> MTCQVTQKAREGTINPIFTCQPAGAQFASIGIKDCIGIVHGGQGCVMFVRLL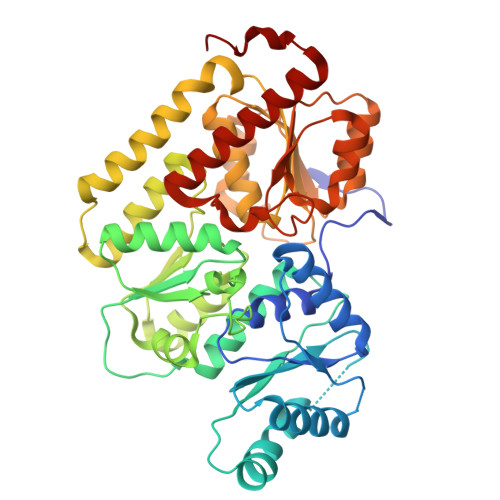ISQHMKESFEIASSSVHEDGAVFGALDRVETAVEVLLTRYPDVKVVPIITTCSTEIIGDDVDGLLSKLEDELLPTKFPGREVHLLTVHCPSFVGSMITGYDKAVHDFVKKFATKDEPSDKINLITGWVNPGDVKELKHLLEVMEVKANVLFEVESFDSPLMPDLEHHSHGSTTIEDLRDTANAKGTIALNRYEGMKAADYLKKKFKVPAVIGPTPVGIRNTDAFLKAVSEMTGQPIPAQLVKERGLALDAIADIGHMFLADKRVAIYANPDLAIGLTEFCLDLEMKPKLLLLGDDNSGYVKDPRVLALQENAPDLEIVTNADFWDLESRIQQGLELDLILGHSKGRFISIDYKVPMVRVGFPTYDRAGMYRHPVLGYGGAMFLAETMANTLFADMEAKKNKEWILNVW> XADVAGTSNRDFRGREQRLFNSEQYNYNNSLNGEVSVWVYAYYSDGSVLVINKNSQYKVGISETFKALKEYYYDPETGTWYNDSYDEYEVNQSIYYPNGGDARKFHSNAKPRAIQIIFSPSVNVRTIKMAKGNAVSVPDEYLQRSHPWEATGIKYRKIKRDGEIVGYSHYFELPHEYNSISLAVSGVHKNPSSYNVGSAHNVMDVFQSCDLALRF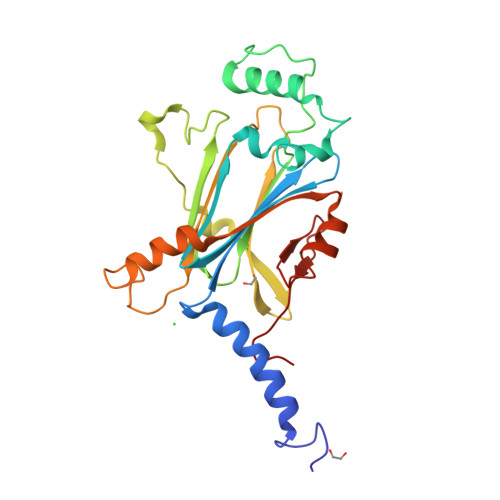CNRYWAELELVNHYISPNAYPYLDINNHSYGVALSNRQ> TTLLNPYFGEFGG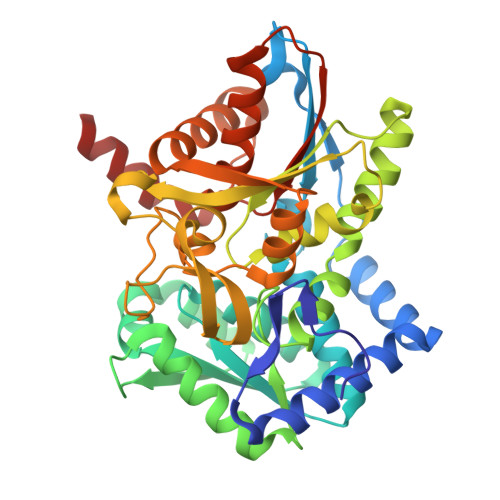MYVPQILMPALNQLEEAFVSAQKDPEFQAQFADLLKNYAGRPTALTKCQNITAGTRTTLYLKREDLLHGGAHKTNQVLGQALLAKRMGKSEIIAETGAGQHGVASALASALLGLKCRIYMGAKDVERQSPNVFRMRLMGAEVIPVHSGSATLKDACNEALADWSGSYETAHYMLGTAAGPHPYPTIVREFQRMIGEETKAQILDKEGRLPDAVIACVGGGSNAIGMFADFINDTSVGLIGVEPGGHGIETGEHGAPLKHGRVGIYFGMKAPMMQTADGQIEESYSISAGLDFPSVGPQHAYLNSIGRADYVSITDDEALEAFKTLCRHEGIIPALESSHALAHALKMMREQPEKEQLLVVNLSGRGDKDIFTVHDILKARGEI> AVLLLGEVTNGALNRDATAKAVAAVKALGDVTVLCAGASAKAAAEEAAKIAGVAKVLVAEDALYGHRLAEPTAALIVGLAGDY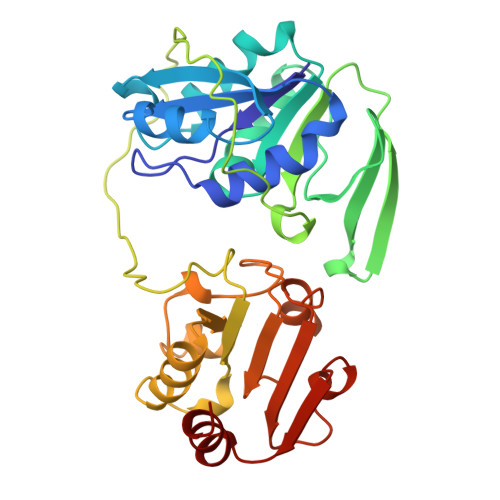SHIAAPATTDAKNVMPRVAALLDVMVLSDVSAILDADTFERPIYAGNAIQVVKSKDAKKVFTIRTASFDAAGEGGTAPVTETAAAADPGLSSWVADEVAESDRPELTSARRVVSGGRGLGSKESFAIIEELADKLGAAVGASRAAVDSGYAPNDWQVGQTGKVVAPELYVAVGISGAIQHLAGMKDSKVIVAINKDEEAPIFQIADYGLVGDLFSVVPELTGKL The most widespread of these mechanisms employs a “controller” (C) protein encoded by a gene downstream of its own promoter, and usually co-transcribed with the endonuclease (R) gene as a single transcriptional unit. The C-protein binds at various sites within the C/R promoter to regulate transcription of its own gene and the associated endonuclease gene. Unusually, in the RM system Esp1396I, the C-protein also represses the MTase (M) gene by binding to the promoter at the transcriptional start site, denoted OM where the C/R genes and the M gene are transcribed convergently from different promoters. Flexibility in this loop is very important for DNA sequence recognition, as it has been observed in the nucleoprotein structures to adopt different conformations depending on which operator site the protein is bound to.

The mutant protein R46A bound with a much lower affinity (∼16 nM), and T36A did not show any measurable binding under these conditions. An even more important role is indicated for T36, since the DNA binding ability of the T36A mutant was completely abolished, as measured by SPR. The ΔΔG for R46A is significantly larger (8.5 kJ mol−1), and that for the T36A mutation must be larger still, since we could not measure any DNA binding activity of this mutant protein. Both R46 and T36 of C.Esp1396I are seen in crystal structures of DNA-protein complexes to interact directly with the base pairs involved in sequence recognition, specifically with the G and C bases, respectively, of the C-box recognition sequence GTC. The T36A mutant structure was observed to adopt two loop conformations (I and III) in equal proportions, indicating the conformational flexibility in this region. T36 is not part of the flexible loop region; it is in fact near the N-terminal end of helix 3 and therefore the likelihood of a mutation at this position altering the loop conformation is minimal. The T36A mutant protein crystal structure showed both the major conformation (I) and the novel conformation observed in this study (III), indicating that both could exist simultaneously in different subunits of the protein dimer. Despite Y37F and T36A only crystallising in the presence of SO4, this anion was not visible in either electron density map. As with the high-resolution wild type structure, the C-terminal tail is also involved in several crystal contacts with multiple monomers in the T36A, Y37F and trigonal R46A structures.

>[2x]GSHMESFLLSKVSFVIKKIRLEKGMTQEDLAYKSNLDRAYISGIERNSRNLTIKSLELIMKGLEVSDVVFFEMLIKEILKHD> MNSGLSRLGIALLAAMFAPALLAADLEKLDVAALPGDRVELKLQFDEPVAAPRGYTIEQPARIALDLPGVQNKLGTKNRELSVGNTRSVTVVEAKDRTRLIINLTALSSYTTRVEGNNLFVVVGNSPHHHHHHHHAGASVASAAPVKASPAPASYAQPIKPKPYVPAGRAIRNIDFQRGEKGEGNVVIDLSDPTLSPDIQEQGGKIRLDFAKTQLPDALRVRLDVKDFATPVQFVNASAQSDRTSITIEPSGLYDYLVYQTDNRLTVSIKPMTTEDAERRKKDNFAYTGEKLSLNFQDIDVRSVLQLIADFTDLNLVASDTVQGNITLRLQNVPWDQALDLVLKTKGLDKRKLGNVLLVAPADEIAARERQELEAQKQIAELAPLRRELIQVNYAKAADIAKLFQSVTSDGGQEGKEGGRGSITVDDRTNSIIAYQPQERLDELRRIVSQLDIPVRQVMIEARIVEANVGYDKSLGVRWGGAYHKGNWSGYGKDGNIGIKDEDGMNCGPIAGSCTFPTTGTSKSPSPFVDLGAKDATSGIGIGFITDNIILDLQLSAMEKTGNGEIVSQPKVVTSDKETAKILKGSEVPYQEASSSGATSTSFKEAALSLEVTPQITPDNRIIVEVKVTKDAPDYQNMLNGVPPINKNEVNAKILVNDGETIVIG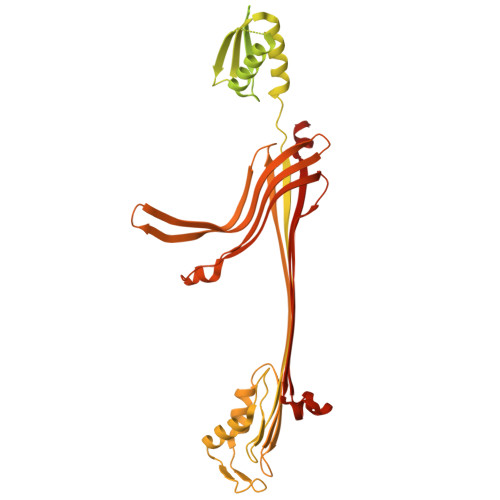GVFSNEQSKSVEKVPFLGELPYLGRLFRRDTVTDRKNELLVFLTPRIMNNQAIAIGRGHHHHHHHH> ECLPGSSPCTDALTCIKADLFCDGEVNCPDGSDEDNKMCATVCDGRFLLTGSSGSFQATHYPKPSETSVVCQWIIRVNQGLSIKLSFDDFNTYYTDILDIYEGVGSSKILRASIWETNPGTIRIFSNQVTATFLIESDESDYVGFNATYTAFNSSELNNYEKINCNFEDGFCFWVQDLNDDNEWERIQGSTFSPFTGPNFDHTFGNASGFYISTPTGPGGRQERVGLLSLPLDPTLEPACLSFWYHMYGENVHKLSINISNDQNMEKTVFQKEGNYGDNWNYGQVTLNETVKFKVAFNAFKNKILSDIALDDISLTYGICNGSLYPEPTLVPTPPPELPTDCGGPFELWEPNTTFSSTNFPNSYPNLAFCVWILNAQKGKNIQLHFQEFDLENINDVVEIRDGEEADSLLLAVYTGPGPVKDVFSTTNRMTVLLITNDVLARGGFKANFTTGYHLGIPEPCKADHFQCKNGECVPLVNLCDGHLHCEDGSDEADCVRFFNGTTNNNGLVRFRIQSIWHTACAENWTTQISNDVCQLLGLGSGNSSKPIFPTDGGPFVKLNTAPDGHLILTPSQQCLQDSLIRLQCNHKSCGKKLAAQDITPK;> IVGGSNAKEGAWPWVVGLYYGGRLLCGASLVSSDWLVSAAACVYGRNLEPSKWTAILGLHMKSNLTSPQTVPRLIDEIVINPHYNRRRKDNAIAMMHLEFKVNYTDYIQPICLPEENQVFPPGRNCSIAGWGTVVYQGTTANILQEADVPLLSNERCQQQMPEYNITENMICAGYEEGGIDSCQGDAGGPLMCQENNRWFLAGVTSFGYKCALPNRPGVYARVSRFTEWIQSFLH;> APFDDDDKIVGGYNCEENSVPYQVSLNSGYHFCGG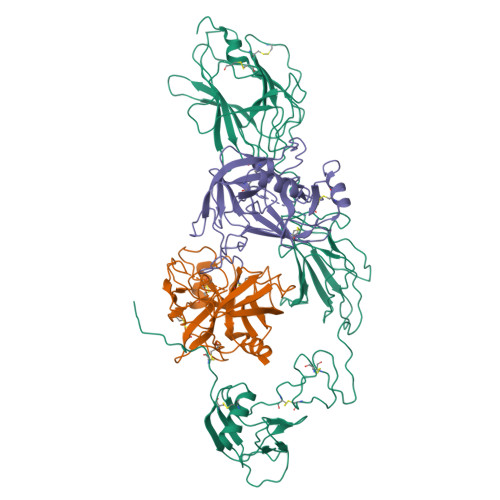SLINEQWVVSAGHCYKSRIQVRLGEHNIEVLEGNEQFINAAKIIRHPQYDRKTLNNDIMLIKLSSRAVINARVSTISLPTAPPATGTKCLISGWGNTASSGADYPDELQCLDAPVLSQAKCEASYPGKITSNMFCVGFLEGGKDSCQGDSGGPVVCNGQLQGVVSWGDGCAQKNKPGVYTKVYNYVKWIKNTIAANS> MIRNFHSLVKRVPRLALTPFFGFRTSMTLADKKLSTGEASVVLAEKIKGITQQNDITEYGTVISIGDGIARVFGLTKVQAGEMVEFKSGIRGMALNLETDNVGVVVLGNDRDIKEGDVVKRTGAIVDVPIGEAMCGRVFDALGNPIDGLGPLKTTQRARVEIKAPGIIPRQSVRQPMQTGIKCVDSLVPIGRGQRELIIGDRQTGKTAIAIDTILNQKEAFNTGDVKKQLYCIYVAVGQKRSTIANLVSILKQHDCMKFTIVVCATASDAAPLQFLAPYSGCAIGEFFRDNGKHALIIYDDLSKQAVAYRQMSLLLRRPPGREAYPGDVFYLHSRLLERAAKMNDSLGGGSLTALPVIETQAGDVSAYIPTNVISITDGQIFLETELFYKGIRPAINVGLSVSRVGSAAQIKAMKKIAGNLKLTLATYRELAAFSQFGSDLDA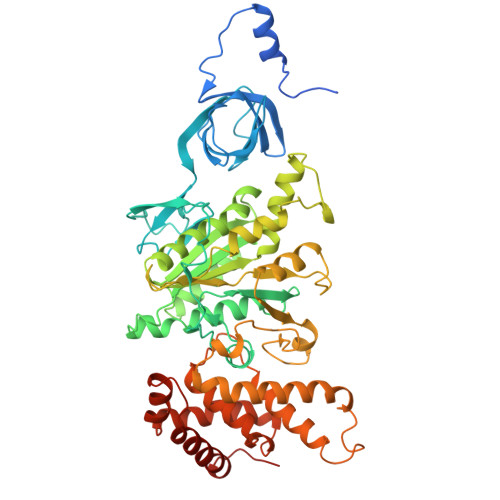KTQQQLNTGERLVEMLKQNQYTPMKVEEQVCIIFAGVKGFLDALVTSEVLKFEKKFLEHVRTNHSALLKRIRDSGDLSEVDTNELNTIIPLFIQEGGFKLKAQ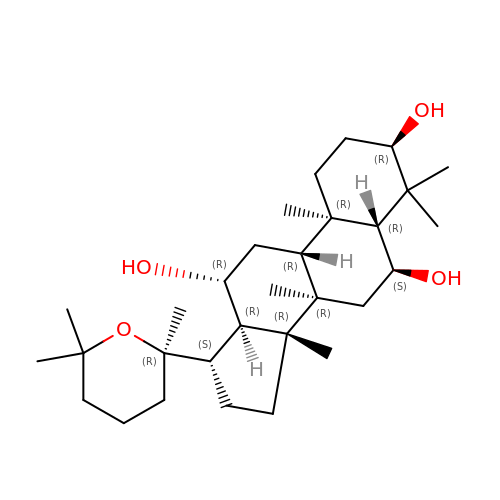(3R,5R,6S,8R,9R,10R,12R,13R,14R,17S)-4,4,8,10,14-pentamethyl-17-[(2R)-2,6,6-trimethyloxan-2-yl]-2,3,5,6,7,9,11,12,13,15,16,17-dodecahydro-1H-cyclopenta[a]phenanthrene-3,6,12-triol | C30 H52 O4 | QFJUYMMIBFBOJY-FAKBLDBGSA-N>SMQRTVARDITLLECVGKGRYGEVWRGSWQGENVAVKIFSSRDEKSWFRETELYNTVMLRHENILGFIASDMTSRHSSTQLWLITHYHEMGSLYDYLQLTTLDTVSCLRIVLSIASGLAHLHIEIFGTQGKPAIAHRDLKSKNILVKKNGQCCIADLGLAVMHSQSTNQLDVGNNPRVGTKRYMAPEVLDETIQVDCFDSYKRVDIWAFGLVLWEVARRMVSNGIVEDYKPPFYDVVPNDPSFEDMRKVVCVDQQRPNIPNRWFSDPTLTSLAKLMKECWYQNPSARLTALRIKKTLTKID[2x]

Members of the transforming growth factor-beta (TGF-β) superfamily bind transmembrane receptor serine/threonine kinases to activate Smad and non-Smad pathways for the control of normal development and tissue repair. Ligand binding induces type II receptor phosphorylation of associated type I receptors, leading to Smad recruitment and phosphorylation by the type I receptor. Most importantly, there is an urgent need for selective ALK2 inhibitors to treat the debilitating bone disorder fibrodysplasia ossificans progressiva (FOP). FOP sufferers carry a gain of function mutation in the intracellular domain of ALK2, resulting in episodic bone formation in skeletal muscle and connective tissue that ultimately renders movement impossible.

To define the mode of action of K02288 we determined its structure in complex with the kinase domain of ALK2 refined at 2.15 Å resolution. The entire chain was traced from residues 202–499, including parts of the L45 loop and activation loop (A-loop) that were previously disordered in the structure of the ALK2-FKBP12 complex (data collection and refinement statistics are provided in Table 1). In particular, the ATP pocket remained occluded by the inhibitory conformations of the A-loop and αC helix, which were stabilized by the hydrogen bond interactions of R375 (A-loop) with S244 (αC), D336 (catalytic loop HRD motif) and D354 (A-loop DLG motif). The 2-aminopyridine of K02288 was bound to the kinase hinge region in an ATP-mimetic fashion with two hydrogen bonds to H284 and H286, respectively. The large trimethoxyphenyl substituent occupied the central pocket area sandwiched between the hydrophobic residues V222, L263, L343 and A353. Two of the three methoxy groups additionally formed a water-mediated hydrogen bond to the catalytic lysine (K235). The solvent channel was occupied by the phenol group, which formed an additional hydrogen bond with D293. Notably, the three methoxy substituents were able to extend more deeply towards the recesses of the pocket periphery, potentially contributing to the high selectivity of K02288. In the crystal structure of the ALK2-K02288 complex this group bound to the exposed solvent channel where substitutions are likely to be well tolerated. Here we report a novel 2-aminopyridine inhibitor K02288 with potent and selective activity against type I BMP receptor kinases.> EEAELAYLLGELAYKLGEYRIAIRAYRIALKRDPNNAEAWYNLGNAYTKQGDYDEAIEYYLRALVLDPNNAEAATNLGQAY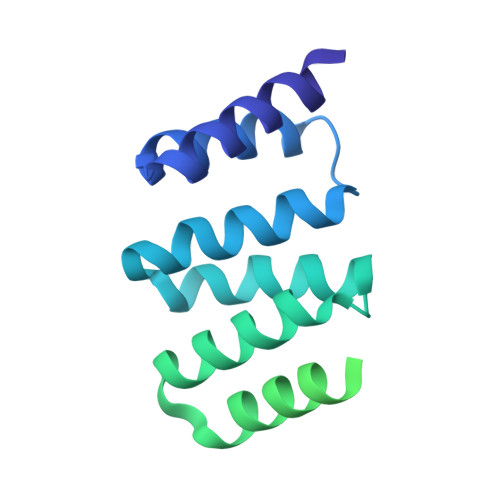MNQGDKDRAKLMLLLALKLDPNNDSARVILGVAKVGIEELAKLASQAQQEGDSEKQKAIELAAEAARVAQEVGDPELEKLALEAARRGDSEKAKAILLAAEAARVAKEVGDPELIKLALEAARRGDSEKARAILEAAERAREAKERGDPEQIKKARELAKR N-{4-[(1E)-N-CARBAMIMIDOYLETHANEHYDRAZONOYL]PHENYL}-1H-INDOLE-3-CARBOXAMIDE | C18 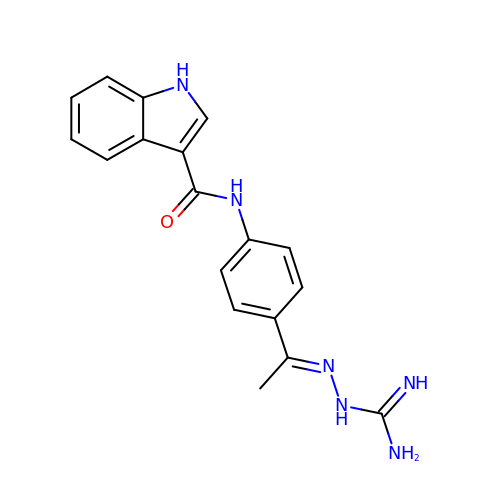H18 N6 O | BTFCNWPQBVODIL-FOKLQQMPSA-N METHYL 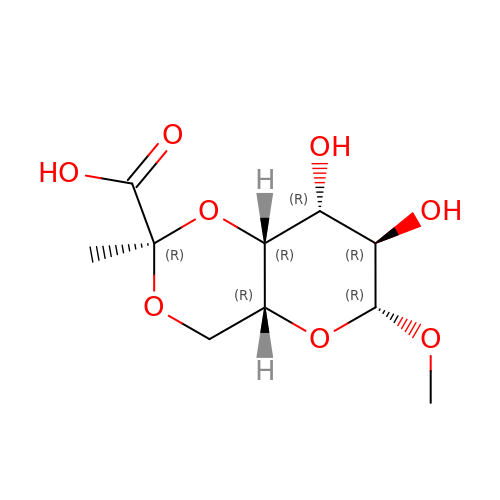4,6-O-[(1R)-1-CARBOXYETHYLIDENE]-BETA-D-GALACTOPYRANOSIDE | C10 H16 O8 | ZDZVLEQWFATHTF-IJWOWSJNSA-N> NAQMGEGRLANYSASGNT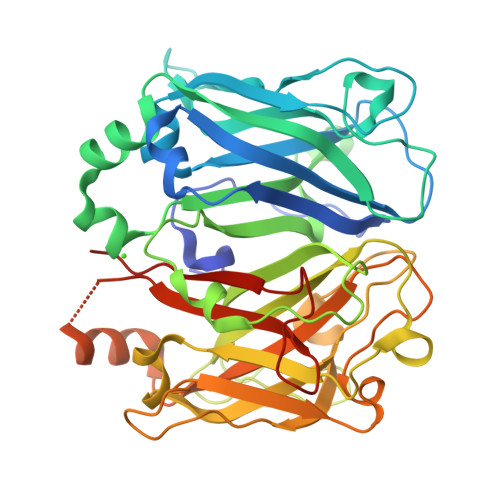FQENPGYTKNYNFSDLQFNPKAITGDVLQGNTIDFEVYGKHNIAASTANWEIRLQLDERLAQYVEKIQVDPKKGVGNSRRTFVRINDSLGRPTNIWKVNYIRANDGLFAGAETTDTQTAPNGVITFEKNLDEIFKEIGADNLKSDRLMYRIYLVSHQDDDKIVPGIESTGYFLTDQDDFYNKLDVSENNSDQFKHGSVNTKYEEANIQTKDGSGSTGANGAIILDHKLTKEKNFSYSTSAKGTPWYANYKIDERLVPYVSGIQMHMVQADKVAYNVAFESGKKVADLAIERREGHENYGMGSITDNDLTKLIDFANASPRPIVVRYVLQLTKPLDEILEEMKAADKIEENAPFGEDFIFDSWLSDTNKKLIQNTYGTGYYYLQDIDGLEVLFQ>GHHHHHHHHHHSSGHIEGRHMKRMIALDGAQGEGGGQILRSALSLSMITGQPFTITSIRAGRAKPGLLRQHLTAVKAATEICGATVEGAELGSQRLLFRPGTVRGGDYRFAIGSAGSCTLVLQTVLPA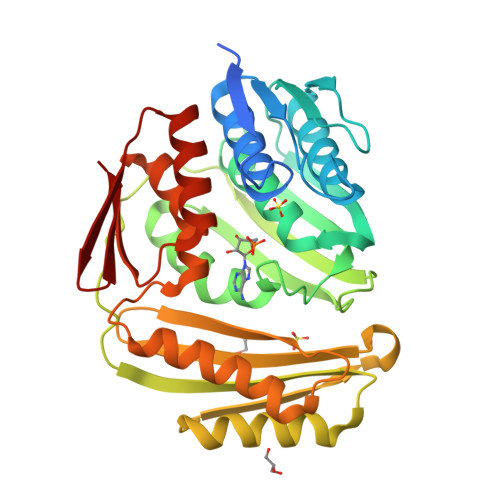LWFADGPSRVEVSGGTDNPSAPPADFIRRVLEPLLAKIGIHQQTTLLRHGFYPAGGGVVATEVSPVASFNTLQLGERGNIVQMRGEVLLAGVPRHVAEREIATLAGSFSLHEQNIHNLPRDQGPGNTVSLEVESENITERFFVVGEKRVSAEVVAAQLVKEVKRYLASTAAVGEYLADQLVLPMALAGAGEFTVAHPSSNLLTNIAVVERFLPVRFSLIETDGVTRVSIE[2x]> MTTITLPALPYGYEDLAPHISKETLEYHHDKHHNTYVVNL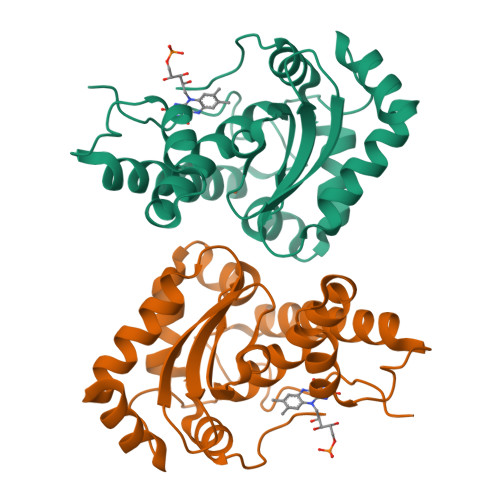NNLIAGTDLEGKTLEEIIKASVGDASKAGIFNNAAQVWNHTFYWNCMAKNGGGKATGALAAKIDEAFGSYEKFAEEFAAAATTQFGSGWAWLVADEVNGKLSIMKTSNADTPLAHGKVAVLTIDVWEHAYYIDFRNARPKYISTFLESLVNWDYANAKYAGQEAGVEK>[8x]MNRLQHIRGHIVSADKHINMSATLLSPLSTHVLNAAQGVPGANMTIVLHRLDPVSSAWNILTTGITNDDGRCPGLITKENFIAGVYKMRFETGKYWDALGETCFYPYVEIVFTIT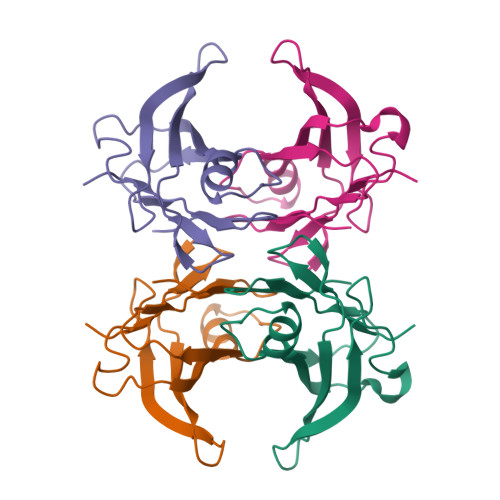NTSQHYHVPLLLSRFSYSTTRGS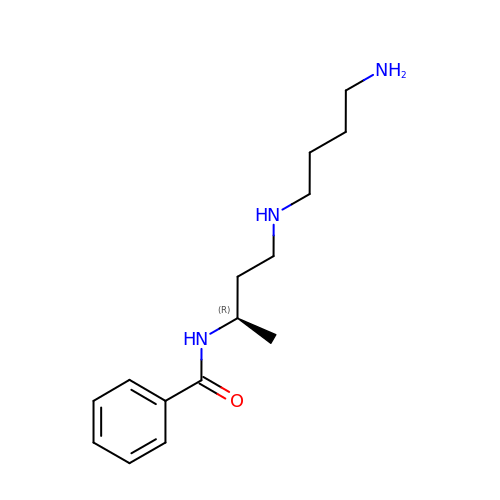N-{(1R)-3-[(4-aminobutyl)amino]-1-methylpropyl}benzamide | C15 H25 N3 O | UWDXTOVSVLCTLF-CYBMUJFWSA-N>MHIIPVASDPKTCSCGVNENSLDFDFTMAFQPIVNCRTKEIFGYEALVRGLNNESAYSVISRVNEDNRYLFDQMCRVKAIALAAKLGLTSKLSINFLPNAIYVPERCIRTTLEAAKRYQFPIENIMFEFTEAE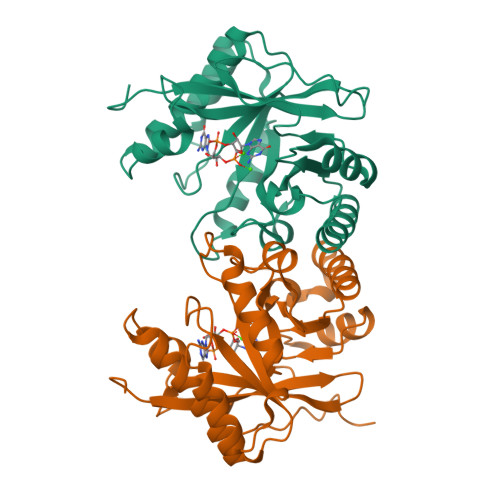RVEDVNHIKRIVEYYKSLGFQTAIDDFGSGYSGLNLLADFQTNIVKVDMGLIRNIHADQVRQSIMKNCLKLFSDLNIQPLAEGVESHAEFAWLKAAGVELMQGYYFAKPGFESLPSVNPEFSEA[4x]>GPLGSPLTASMLASAPPQEQKQMLGERLFPLIQAMHPTLAGKITGMLLEIDNSELLHMLESPESLRSKVDE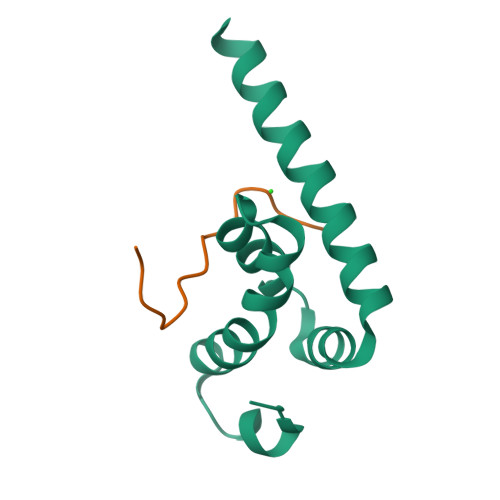AVAVLQAHQAKEAAQKA[2x];>SNLNPNAAEFVPGVKYG[2x]Here we report protein crystal structures of a piscine betanodavirus, the Grouper nervous necrosis virus (GNNV), in four different forms. The overall topological structure of the GNNV CP consists of the N-terminal arm (N-arm) (residues 34−51), the shell domain (S-domain) (residues 52−213), the linker region (residues 214−220) and the protrusion domain (P-domain) (residues 221−338). The S-domain comprises an eight-stranded anti-parallel β-sandwich with three short α-helices, which is a canonical structural feature similar to other virus CPs. The P-domain folds into an independent structure, including eight anti-parallel β-strands and a short α-helix connected with loops of various lengths.

In the delta-P-domain mutant, sixty copies of the S-domain assemble with interactions of I2, I3 and I5 symmetries into a T = 1 SVP with a diameter ~190 Å. Only residues 52−214 of each subunit are observed at a resolution of 3.1 Å. As expected, the delta-P-domain mutant comprises a canonical eight-stranded anti-parallel β-sandwich with three short α-helices similar to the S-domain of T = 3 GNNV-LP. Although the organization of the equivalent subunits around the I3 axes of the T = 1 delta-P-domain mutant is notably similar to the arrangement of the iASU subunits of the T = 3 GNNV-LP, the organization of the trimeric subunits is flatter than that of the T = 3 GNNV-LP. In the T = 1 delta-P-domain mutant, there is no Ca2+ observed at corresponding calcium-binding sites as seen in the S-domain of T = 3 GNNV-LP. The hollow or empty binding site exhibits an expanded geometry with maximum movement of ~2.6 Å of the main chains. We find that, without the Ca2+-mediated interactions at the subunit interfaces, the weaker contacts cause changes in the inter-subunit organization, with expanded assembly of the T = 1 delta-P-domain mutant, similar to the structure in the Asp mutants of T = 1 SeMV. However, the bent conformation of the subunit dimer leads to the disordered N-arm lying at the inner cavity of the T = 1 delta-P-domain mutant without β-annulus formation. The T = 1 delta-P-domain mutant without Ca2+ incorporated shows that the region containing the residues that potentially coordinate Ca2+ exhibits an expanded geometry, decreasing subunit contacts along the two-, three- and five-fold axes, and a flatter dimeric contact of curvature ~155°, compared with T = 3 GNNV-LP.

>TDAPVSKASTVTGFGRGTNDVHLSGMSRISQAVLPAGTGTDGYVVVDATIVPDLLPRLGHAARIFQRYAVETLEFEIQPMCPANTGGGYVAGFLPDPTDNDHTFDALQATRGAVVAKWWESRTVRPQYTRTLLWTSSGKEQRLTSPGRLILLCVGNNTDVVNVSVLCRWSVRLSVPSLENPEE[60x]(S)-2-AMINO-3-(5-TERT-BUTYL-3-(PHOSPHONOMETHOXY)-4-ISOXAZOLYL)PROPIONIC ACID | C11 H19 N2 O7 P | 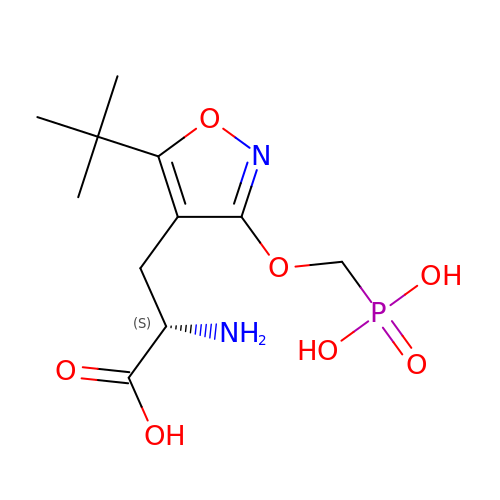AGSOOCUNMTYPSE-ZETCQYMHSA-N>KHTTIGFKIDRPHDKVLSSVLKNKLSTYVKESFKFFKSGYAQKGYLGSENDSIELDDVANLMFYGEGQIGTNKQPFMFIFDTGSANLWVPSVNCDSIGCSTKHLYDASASKSYEKDGTKVEISYGSGTVRGYFSKDVISLGDLSLPYKFIEVTDADDLEPIYSGSEFDGILGLGWKDLSIGSIDPVVVELKKQNKIDNALFTFYLPVHDKHVGYLTIGGIESDFYEGPLTYEKLNHDLYWQIDLDIHFGKYVMQKANAVVDSGTSTITAPTSFLNKFFRDMNVIKVPFLPLYVTTCDNDDLPTLEFHSRNNKYTLEPEFYMDPLSDIDPALCMLYILPVDIDDNTFILGDPFMRKYFTVFDY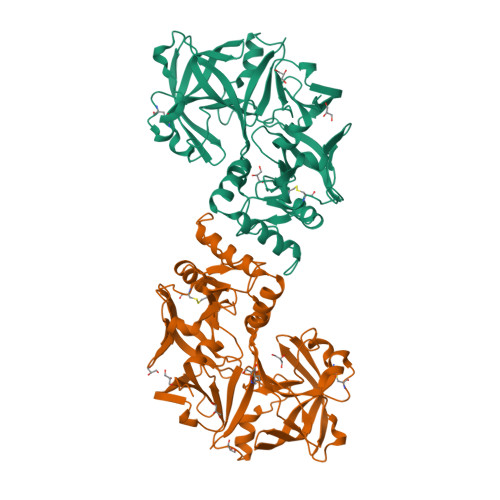EKESVGFAVAKNL[2x]> GAMKKVEILMVVDAAAALASRDLQSNIYLIDTNKYMGSGNEGQAELKTACKDGQLLCWRVVAISPDNEVDIVEFNGQMINDRVCIPT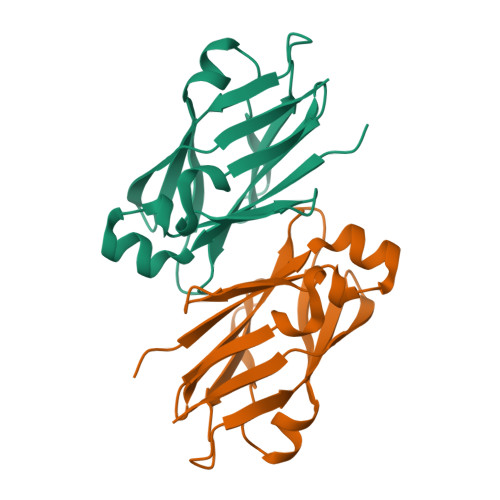KQGLSGDEFWEGRVEAQGQASTQQYNATLSIDGSRLTFDPFLVISL Analogous to characteristic antimicrobial polymorphic toxins of Gram-negative bacteria, the LXG proteins consist of a conserved N-terminal domain (LXG), a middle domain of variable length, and a C-terminal variable toxin domain. We show here that LXG proteins transit the Esx secretion system of Streptococcus intermedius (Si) and function as antibacterial toxins that mediate contact-dependent interspecies antagonism. The genome of SiB196 encodes two additional LXG proteins, which we named TelA and TelC. We discovered that TelC, a protein lacking characterized homologs, adopts a previously unobserved fold and catalyzes degradation of the cell wall precursor molecule lipid II.

To gain further insight into TelC function, we determined the crystal structure of TelCtox to 2.0 Å resolution. The structure of TelCtox represents a new fold; it is comprised of distinct and largely α-helical N- and C-terminal lobes. The single β element of TelCtox is a hairpin that protrudes from the N-terminal lobe. Although TelCtox does not share significant similarity to previously determined structures, we located its putative active site within a shallow groove that separates the N- and C-terminal lobes. This region contains a calcium ion bound to several residues that comprise the conserved aspartate-rich motif. The substrates may be inaccessible or TelC could be inactive in the cytoplasm. It is worth noting that TelC contains a calcium ion bound at the interface of its N- and C-terminal lobes. Analysis of the reaction products showed that TelCtox cleaves lipid II – severing the molecule at the phosphoester linkage to undecaprenyl. Our experiments showed that TelCtox is capable of hydrolyzing cleaved undecaprenyl derivatives but displays a strict requirement for the pyrophosphate group, indicating the potential for TelC to simultaneously disrupt two critical Gram-positive cell wall polymers. S. aureus cells expressing extracellularly-targeted TelCtox exhibited significantly reduced viability, and when examined microscopically, displayed a cessation of cell growth followed by lysis that was not observed in control cells. Consistent with its ability to inhibit a conserved step in peptidoglycan biosynthesis, TelC exhibited toxicity towards diverse Gram-positive species including Si, S. aureus and E. faecalis.

> MGSSHHHHHHSQDPSDLSWSKRLSAYAALKDLTLSKQDKVFLEHLMTEYGFDSTTARQILKLKQGLERKFSSIFDDYTQEERDYLLFRIIGSVSYNGVKWDETAGYLSRYFYKEVVSNPVTGEKQKVPKSLLDIFQELGLSKAEAKQLQYNLSLQHEMAGGTLSTTGDMVKQDPDYYETAKNSYKLVYGTTEGFDKFWDERLKAYSNDGRGNADFTHQSITMATHLNPTSVQLSDIYGGRKHVKNLAGWEGDTTYNANERKPSIGEDDYKADLDSVNIIGRMKKGQSYQSAMSSYYSDVQKGHSVREKEFLKNKDWEKVKKTIYDSLVPNGINKNADSVVKDYIAKNYPDVSKFLSRLESVAGGQ> GGDPHMMFGKKKNNGGSSTARYSAGNKYNTLSNNYALSAQQLLNASKIDDIDSMMGFERYVPPQYNGRFDAKDIDQIPGRVGWLTNMHATLVSQETLSSGSNGGGNSNDGERVTTNQGISGVDFYFLDEEGGSFKSTVVYDPYFFIACNDESRVNDVEELVKKYLESCLKSLQIIRKEDLTMDNHLLGLQKTLIKLSFVNSNQLFEARKLLRPILQDNANNNVQRNIYNVAANGSEKVDAKHLIEDIREYDVPYHVRVSIDKDIRVGKWYKVTQQGFIEDTRKIAFADPVVMAFDIETTKPPLKFPDSAVDQIMMISYMIDGEGFLITNREIISEDIEDFEYTPKPEYPGFFTIFNENDEVALLQRFFEHIRDVRPTVISTFNGDFFDWPFIHNRSKIHGLDMFDEIGFAPDAEGEYKSSYCSHMDCFRWVKRDSYLPQGSQGLKAVTQSKLGYNPIELDPELMTPYAFEKPQHLSEYSVSDAVATYYLYMKYVHPFIFSLCTIIPLNPDETLRKGTGTLCEMLLMVQAYQHNILLPNKHTDPIERFYDGHLLESETYVGGHVESLEAGVFRSDLKNEFKIDPSAIDELLQELPEALKFSVEVENKSSVDKVTNFEEIKNQITQKLLELKENNIRNELPLIYHVDVASGYPNIMTTNRLQPDSIKAERDCASCDFNRPGKTCARKLKWAWRGEFFPSKMDEYNMIKRALQNETFPNKNKFSKKKVLTFDELSYADQVIHIKKRLTEYSRKVYHRVKVSEIVEREAIVCQRENPFYVDTVKSFRDRRYEFKGLAKTWKGNLSKIDPSDKHARDEAKKMIVLYDSLQLAHKVILNSFYGYVMRKGSRWYSMEMAGITCLTGATIIQMARALVERVGRPLELDTDGIWCILPKSFPETYFFTLENGKKLYLSYPCSMLNYRVHQKFTNHQYQELKDPLNYIYETHSENTIFFEVDGPYKAMILPSSKEEGKGIKKRYAVFNEDGSLAELKGFELKRRGELQLIKNFQSDIFKVFLEGDTLEGCYSAVASVCNRWLDVLDSHGLMLEDEDLVSLICENRSMSKTLKEYEGQKSTSITTARRLGDFLGEDMVKDKGLQCKYIISSKPFNAPVTERAIPVAIFSADIPIKRSFLRRWTLDPSLEDLDIRTIIDWGYYRERLGSAIQKIITIPAALQGVSNPVPRVEHPDWLKRKIAT

The Saccharomyces cerevisiae B-family replicative DNA polymerases, namely Pol ϵ, Pol δ and Pol α, have been estimated to incorporate about 13 000 NTPs during each cell cycle of the yeast genome, and Pol ϵ seems to incorporate the majority of NTPs, roughly four times as many ribonucleotides as Pol δ. Other examples where an amino acid adjacent to the steric gate residue influences ribonucleotide discrimination are found among B-family polymerases. It was first shown in the ϕ29 DNA polymerase that B-family polymerases have a conserved tyrosine (Y645 in Pol ϵ) that functions as a steric gate. Our data show that Pol ϵ discriminates NTPs through the concerted action of a steric gate residue (Y645) and a sensor in the finger domain (N828). A comparison with other B-family DNA polymerases showed that both Y645 and N828 are structurally conserved residues, thus reinforcing their functional importance.

Previous biochemical experiments showed that M644GPol ϵ has an increased propensity to incorporate NTPs, suggesting that M644GPol ϵ might more easily accommodate a ribonucleotide in the active site. A series of crystal structures were determined of M644GPol2CORE (the catalytic domain of Pol ϵ (136 kDa)) in complex with dTTP or UTP and dCTP or CTP opposite the template dA and dG, respectively. The two structures of M644GPol2CORE-UTP and M644GPol2CORE-CTP aligned well in the polymerase active site when the two structures were superimposed. In both structures, the NTPs adopted the same C3’-endo conformation, and the 3′-dideoxy end of the primer terminus was at the same distance from the α-phosphate of the incoming nucleotide as found in structures with a dNTP. Thus, the NTPs were in a position admissible for chemistry to occur if a 3′-OH group were to be present at the DNA primer terminus. The described structural changes were also found when comparing M644GPol2CORE-CTP with M644GPol2CORE-dCTP. However, a small ∼1Å shift in the backbone Cα-atom of the catalytic residue D877 towards the cavity between D877 and Y645 was consistently observed in all M644GPol2CORE structures when compared to wild-type Pol2CORE structures. Here, the M644GPol ϵ variant allowed us to solve the first high-resolution structures of a B-family polymerase with a ribonucleotide in the polymerase active site. Instead, N828 in the finger domain, positioned on the opposite side of the nucleotide (not facing the 2′-OH), had moved 3.1 Å and a loose hydrogen bond with the β-phosphate was disrupted.> SQAGDTLNDVIQDPTRRNKLINDNNLLKGIIMGRDGPVPSSRELIVRPDTLRAIINNRATIETTTMKSMYTSSRYLFPQGRIDFTTPDSGFDDVIKLSPQFTSGVQAALAKATGTEKREALQNLFQEYGHVFRTKVHIGGVLSAHTMETFSKLNVKYIVNGGDYTKIQNTEEWVASTNQSEHWRVIEVTEVTAVADLLPQPIRGQVKDLLKPLLGKWVDVEKVPGLESLPVSVYRPKGAIPAGWFWLGDTADASKALLVKPTLPARSGRNPALTSLHQGSGMTEQPFVDLPQYQYLSTYFGSFAHDTPP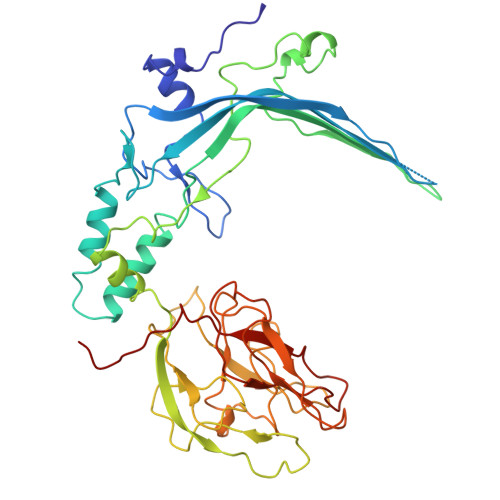GSTLRGLRPDHVLPGRYEMHGDTISTAVYVTRPVDVPFPEDECFDLKSLVRVKLPGSGNPPKPRSALKKSMVLFDSGEK>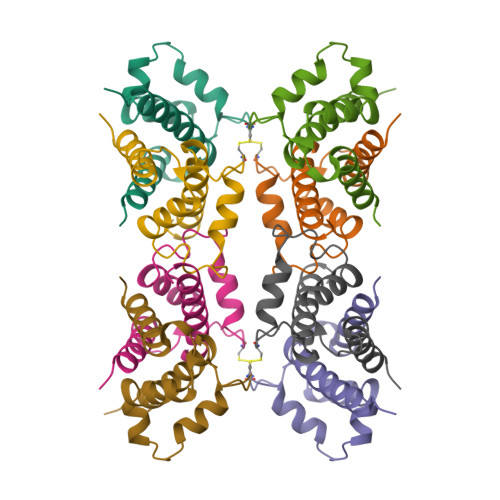[2x]PSQMEHAMETMMFTFHKFAGDKGYLTKEDLRVLMEKEFPGFLENQKDPLAVDKIMKDLDQCRDGKVGFQSFFSLIAGLTIACNDYFVVHMKQKGKK Some bacteria express a binary toxin translocation system, consisting of an enzymatic subunit and translocation pore, that delivers enzymes into host cells through endocytosis. The B-components of the C. perfringens, C. difficile, and C. spiroforme systems bind to the host cell’s lipolysis-stimulated lipoprotein receptor (LSR), after which the A–B complex is internalized by endocytosis. Then, the A-component is translocated via the B-component pore across the endosomal membrane into the cytosol, assisted by host-cell chaperones, including Hsp90 and Hsp70. In the cytosol, the A-component covalently transfers an ADP-ribose to actin, causing F-actin depolymerization, cell rounding, and eventually cell death.

Here, we report two cryo-EM structures of the CDTa-bound CDTb-pore, long and short, at 2.64- and 2.56-Å resolution, respectively. We describe the interaction between CDTa and CDTb based on the highest-resolution structure to date of the CDTa-bound CDTb-pore (short). By contrast, the short structure showed no density at the tip of the β-barrel stem (residues 332–363) because of its flexibility. The most striking difference between the structures was that D4II (receptor-binding domain II) was observed in the long, but not in the short complex. Binding induces the unfolding and tilting of the first N-terminal α-helix of CDTa, in addition to conformational changes to one of the constriction sites in the CDTb-pore, called the NSS-loop, which grips CDTa. Our 2.56-Å resolution analysis provided more precise insights, revealing ‘in’ and ‘out’ loop conformations (blue and yellow, respectively). In the A, B, and G subunits, which had almost no interaction with the CDTa via the NSS-loop, the loop had two clear conformations. In the D and E subunits, the NSS-loop showed two conformations. However, in the C and F subunits, the NSS-loop was only observed in the ‘out’ conformation because of steric hindrance from CDTa. (3) Two NSS-loop conformations would adapt to fit transient translocational CDTa states: the unfolded and folded complexes showed different ‘in’ and ‘out’ conformations in the subunit D NSS-loop. The short CDTa-bound CDTb-pore map represents the total map, showing the small differences between folded and unfolded CDTa.

>NNNFFDPKLMSDWEDEDLDTDNDNIPDSYERNGYTIKDLIAVKWEDSFAEQGYKKYVSNYLESNTAGDPYTDYEKASGSFDKAIKTEARDPLVAAYPIVGVGMEKLIISTNEHASTDQGKTVSRATTNSKTESNTAGVSVNVGYQNGFTANVTTNYSHTTDNSTAVQDSNGESWNTGLSINKGESAYINANVRYYNTGTAPMYKVTPTTNLVLDGDTLSTIKAQENQIGNNLSPGDTYPKKGLSPLALNTMDQFSSRLIPINYDQLKKLDAGKQIKLETTQVSGNFGTKNSSGQIVTEGNSWSDYISQIDSISASIILDTENESYERRVTAKNLQDPEDKTPELTIGEAIEKAFGATKKDGLLYFNDIPIDESCVELIFDDNTANKIKDSLKTLSDKKIYNVKLERGMNILIKTPTYFTNFDDYNNYPSTWSNVNTTNQDGLQGSANKLNGETKIKIPMSELKPYKRYVFSGYSKDPLTSNSIIVKIKAKEEKTDYLVPEQGYTKFSYEFETTEKDSSNIEITLIGSGTTYLDNLSITELNSTPEILDEPEVKIPTDQEIMDAHKIYFADLNFNPSTGNTYINGMYFAPTQTNKEALDYIQKYRVEATLQYSGFKDIGTKDKEMRNYLGDPNQPKTNYVNLRSYFTGGENIMTYKKLRIYAITPDDRELLVLSVD[7x];> APIERPEDFLKDKEKAKEWERKEAERIEQKLERSEKEALESYKKDSVEISKYSQTRNYFYDYQIEANSREKEYKELRNAISKNKIDKPMYVYYFESPEKFAFNKVIRTENQNEISLEKFNEFKETIQNKLFKQDGFKDISLYEPGKGDEKPTPLLMHLKLPRNTGMLPYTNTNNVSTLIEQGYSIKIDKIVRIVIDGKHYIKAEASVVSSLDFKDDVSKGDSWGKANYNDWSNKLTPNELADVNDYMRGGYTAINNYLISNGPVNNPNPELDSKITNIENALKREPIPTNLTVYRRSGPQEFGLTLTSPEYDFNKLENIDAFKSKWEGQALSYPNFISTSIGSVNMSAFAKRKIVLRITIPKGSPGAYLSAIPGYAGEYEVLLNHGSKFKINKIDSYKDGTITKLIVDATLIPENLYFQGLEHHHHHH> DYKDDDDKMPGGLEALRALPLLLFLSYACLGPGCQALRVEGGPPSLTVNLGEEARLTCENNGRNPNITWWFSLQSNITWPPVPLGPGQGTTGQLFFPEVNKNHRGLYWCQVIENNILKRSCGTYLRVRNPVPRPFLDMGEGTKNRIITAEGIILLFCAVVPGTLLLFRKRWQNEKFGRSIATRSMFKGIVEGIGIIEKIDIYTDLDKY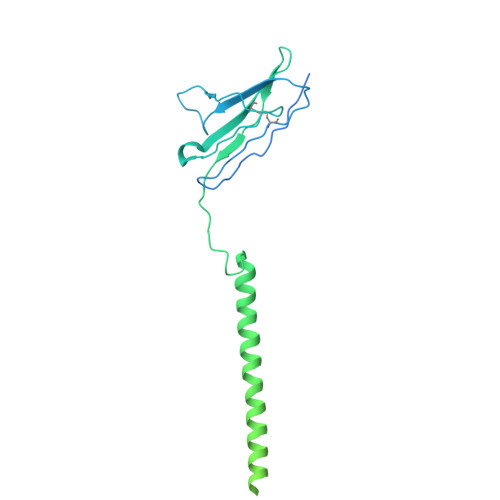AIRFPENMLNGIKKESSIMFNGCFLTVTSVNSNIVWFDIFEKEARKLDTFREYKVGDRVNLGTFPKFGAASGGHILSARISCVASIIEIIENEDYQQMWIQIPENFTEFLIDKDYIAVDGISLTIDTIKNNQFFISLPLKIAQNTNMKWRKKGDKVNVELSNKINANQCW> MDPPARKEKTKVKESVSRVEKAKQKSAQQELKQRQRAEIYALNRVMTELEQQQFDEFCKQMQP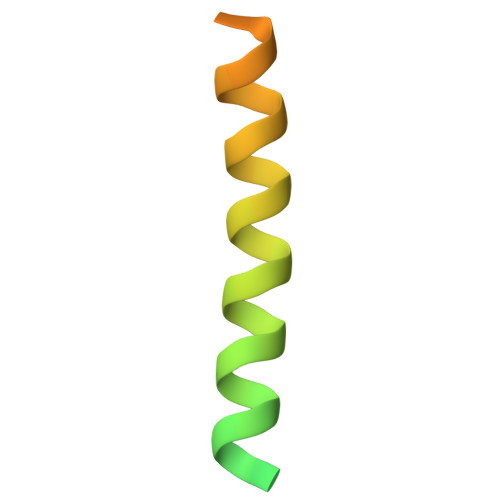PGE>ENLYFQGKTVVFVYKDTLKSYKEKFLLKIEKDLKNHHEYYTLKLDDLSEVVEILEENSRICCIVLDRASFNIEAFHNIAHLNTKLPIFVASDYSQSIKLNLRDFNLNINFLQYDALAGEDSDFIHKTITNYFNDILPPLTYELFKYSKSFNSAFCTPGHQGGYGFQRSAVGALFYDFYGENIFKTDLSISMKELGSLLDHSEAHKDAEEYISKVFKSDRSLIVTNGTSTANKIVGMYSVADGDTILVDRNCHKSVTHLMMMVDVNPIYLKPTRNAYGIIGGIPKKEFKRETIQEKIDNSNIADKWPEYAVVTNSTYDGILYNTDTIHRELDVKKLHFDSAWIPYAIFHPIYKHKSAMQIEPRPEHIIFETQSTHKLLAAFSQSSMLHIKGDYNEEVLNEAFMLHTSTSPFYPIVASVETAAAMMEGEQGYNLIDKTINLAIDFRRELIKLRSEANGWFFDVWQPDNISNKEAWLLRNADKWHGFKNVDGDFLSLDPIKITILTPGIKDNDVQDWGVPADVVAKFLDEHDIVVEKSGPYSLLFIFSLGTTKAKSVRLISVLNKFKQMYDENTLVEKMLPTLYAEDPKFYEDMRIQEVSERLHQYMKEANLPNLMYHAFNVLPEQQLNPHRAFQKLLKGKVKKVPLAELYEHTSAVMILPYPPGIPVIFPGEKITEESKVILDFLLMLEKIGSMLPGFDTDIHGPERAKDGKLYIKVID[5x]

A previous report showed that a F. novicida transposon mutant with insertions in cadA (FTT_0406), which encodes a putative aspartate aminotransferase fold (AAT-fold) pyridoxal 5′-phosphate (PLP)-dependent lysine decarboxylase (hereafter referred to as LdcF), was attenuated in mouse spleen. Bacterial AAT-fold PLP-dependent basic amino acid decarboxylases are grouped into a superfamily termed LAOdc because these enzymes decarboxylate lysine (LdcI, LdcC and LdcA), arginine (AdcI) and ornithine (OdcI and OdcC) into corresponding polyamines (cadaverine, agmantine and putrescine) while consuming protons and producing CO2. LdcF sequences found in Francisellaceae strains display a high level of sequence identity (83%), and contain four functional regions, corresponding to a wing domain (Pfam ID: PF03709), a PLP-binding domain and a AAT-like domain (both corresponding to Pfam ID: PF01276), and a C-terminal domain (Pfam ID: PF03711). It uncovers the important role of this previously uncharacterized protein in survival in the host cells through participation in oxidative stress response, thereby identifying LdcF as a potential drug target.

We were able to determine the structure of F. novicida LdcF from X-ray diffraction data collected to a resolution of 3.4 Å. In agreement with the relationship between LdcF and LdcI families disclosed by the phylogenetic analysis and the relatively high level of sequence conservation, structural alignment between F. novicida LdcF and E. coli LdcI dimers extracted from their respective decameric crystal structures demonstrates a high overall similarity, with a root-mean-square-deviation (RMSD) of 1.043 Å over 1,223 aligned atoms. Like LdcI and other LAOdcs, the LdcF monomer is organized in three different structural domains: A N-terminal wing domain involved in stabilization of the ring assembly though inter-dimer contacts (residues 1–130), a central core domain which contains a covalently bound PLP cofactor (residues 131–564) and a C-terminal domain (residues 565–713), which partially constitutes an entry channel into the active site. The core domain encompasses a linker region (residues 113–184), a PLP-binding domain consisting of a seven-stranded β-sheet surrounded by eight α-helices (residues 185–419), and an AAT-like domain which harbors an antiparallel four-stranded β-sheet and three α-helices near the dimerization interface (residues 420–564). While the overall structures of LdcF and LdcI are very similar, some notable differences were found in both the AAT-like and the C-terminal domains. Moreover, a comparison of the ppGpp binding pocket in LdcI with the equivalent region in LdcF revealed that, despite the overall high sequence conservation, only two out of 10 ppGpp-interacting residues are conserved between the two proteins.>MGSSHHHHHHSSGRENLYFQGMPSLTPRCIIVRAGQTEWSKSGQYTGLTDLPLTPYGEGQMLRTGESVFRNNQFLNPDNITYIFTSPRLRARQTVDLVLKPLSDEQRAKIRVVVDDDLREWEYGDYEGMLTREIIELRKSRGLDKERPWNIWRDGCENGETTQQIGLRLSRAIARIQNLHRKHQSEGRASDIMVFAHGHALRYFAAIWFGLGVQKKCETIEEIQNVKSYDDDTVPYVKLESYRHLVDNPCFLLDAGGIGVLSYAHHNIDEPALELAGPFVSPPEEESQHGDV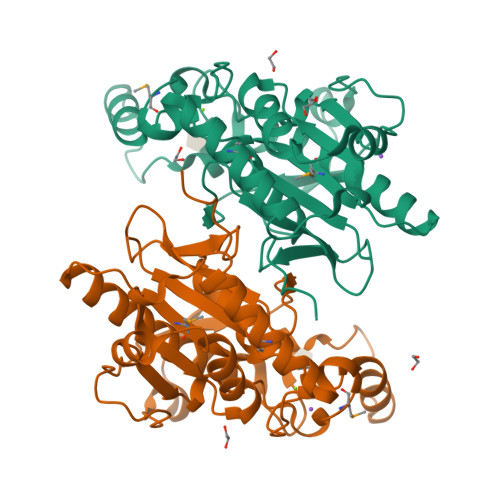[4x]> GPDSMASVTLSEAEKVYIVHGVQEDLRVDGRGCEDYRCVEVETDVVSNTSGSARVKLGHTDILVGVKAEMGTPKLEKPNEGYLEFFVDCSASATPEFEGRGGDDLG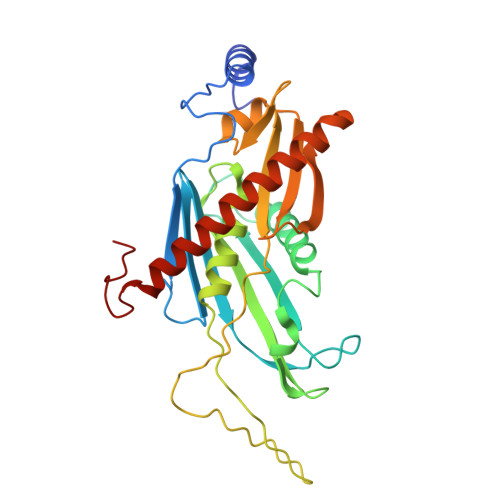TEIANTLYRIFNNKSSVDLKTLCISPREHCWVLYVDVLLLECGGNLFDAISIAVKAALFNTRIPRVRVLEDEEGSKDIELSDDPYDCIRLSVENVPCIVTLCKIGYRHVVDATLQEEACSLASLLVSVTSKGVVTCMRKVGKGSLDPESIFEMMETGKRVGKVLHASLQSVVHKEESLGPKRQKVGFLG> GHMNAYDAYMKEIAQQMRGELTQNGFTSLETSEAVSEYMNQVNADDTTFVVINSTCGCAAGLARPAAVAVATQNEHRPTNTVTVFAGQDKEATATMREFIQQVPSSPSYALF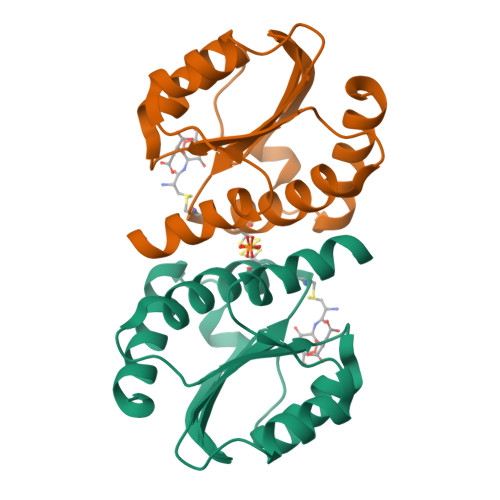KGRDLVYFMPREFIEGRDINDIAMDLKDAFDENCK> MIGKKSFQTNVYRMSKFDTYIFNNLYINDYKMFWIDSGIAKLIDKNCLVSYEINSSSIILLKKNSIQRFSLTSLSDENINVSVITISDSFIRSLKSYILGDLMIRNLYSENKDLLLWNCEHNDIAVLSEVVNGFREINYSDEFLKVFFSGFFSKVEKKYNSIFITDDLDAMEKISC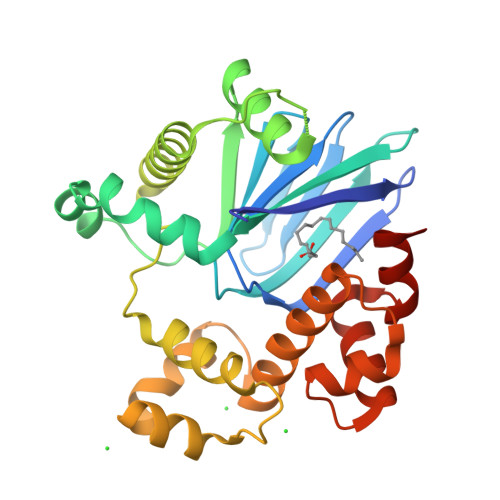LVKSDITRNWRWADICGELRTNRMILKKELESRGVKFRELINSIRISYSISLMKTGEFKIKQIAYQSGFASVSYFSTVFKSTMNVAPSEYLFMLTGVAEK> GSSVVVDTNGQPVSNGADAYYLVPVSHGHAGLALAKIGNEAEPRAVVLDPHHRPGLPVRFESPLFINIIKESYFLNIKFGPSSSDSGVWDV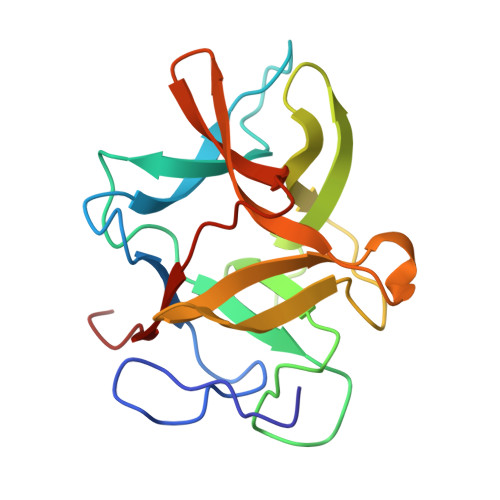IQQDPIGLAVKVTDTKSLLGPFKVEKEGEGYKIVYYPERGQTGLDIGLVHRNDKYYLAVKDGEPCVFKIRKATDE> MSRSTVFGPGSLY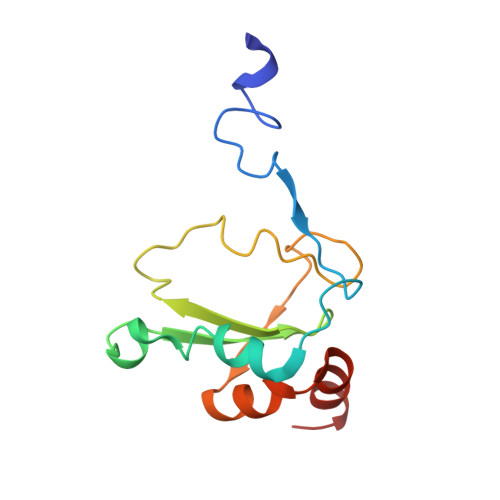SFTKFGSFNRSPTNCTLNKRMKDIFRLENQKHIRNDFDRERRYRMCTKCGITTVTINFNNVPSARVGLWGRCADDKDYTHHRMVDITQREYEVLRESPVEKRLNWWRYER> ARASPGSAASPRLREGPELSPDDPAGLLDLRQGMFAQLVAQNVLLIDGPLSWYSDPGLAGVSLTGGLSYKEDTKELVVAKAGVYYVFFQLELRRVVAGEGSGSVSLALHLQPLRSAAGAAALALTVDLPPASSEARNSAFGFQGRLLHLSAGQRLGVHLHTEARARHA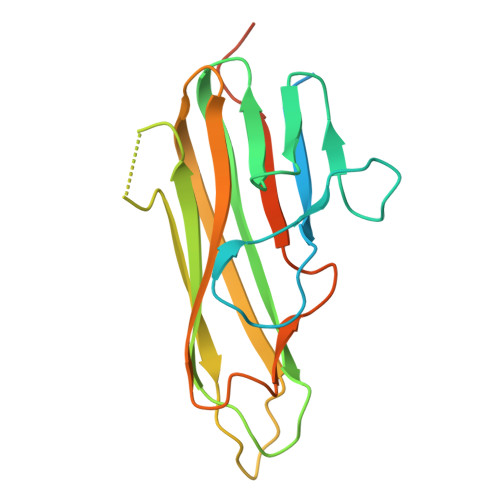WQLTQGATVLGLFRVTPEIPAGLPSPRSEHHHHHH> TTCTTCTTC;> 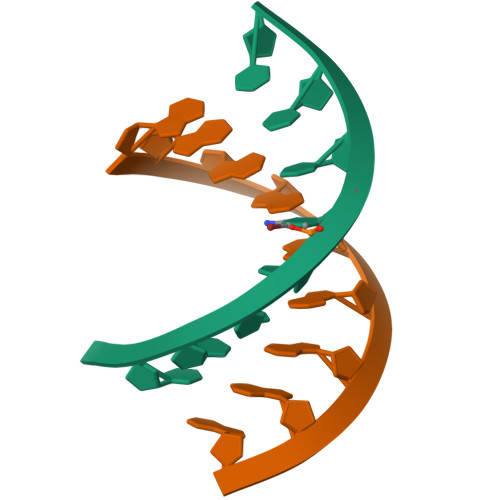GAAGAAGAA> MTTLRAFTCDDLFRFNNINLDPLTETYGIPFYLQYLAHWPEYFIVAEAPGGELMGYIMGKAEGSVAREEWHGHVTALSVAPEFRRLGLAAKLMELLEEISERKGGFFVDLFVRVSNQVAVNMYKQLGYSVYRTVIEYYSASNGEPDEDAYDMRKALSRDTEKKSIIPLPHPVRPEDIE;> MATRGHVQDPNDRRLRPIYDYLDNGNNKMAIQQADKLLKKHKDLHCAKVLKAIGLQRTGKQEEAFTLAQEVAALEPTDDNSLQALTILYREMHRPELVTKLYEAAVKKVPNSEEYHSHLFMAYARVGEYKKMQQAGMALYKIVPKNPYYFWSVMSLIMQSISAQDENLSKTMFLPLAERMVEKMVKEDKIEAEAEVELYYMILERLGKYQEALDVIRGKLGEKLTSEIQSRENKCMAMYKKLSRWPECNALSRRLLLKNSDDWQFYLTYFDSVFRLIEEAWSPPAEGEHSLEGEVHYSAEKAVKFIEDRITEESKSSRHLRGPHLAKLELIRRLRSQGCNDEYKLGDPEELMFQYFKKFG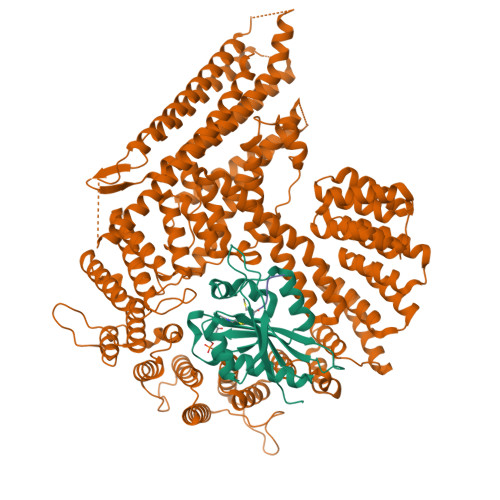DKPCCFTDLKVFVDLLPATQCTKFINQLLGVVPLSTPTEDKLALPADIRALQQHLCVVQLTRLLGLYHTMDKNQKLSVVRELMLRYQHGLEFGKTCLKTELQFSDYYCLLAVHALIDVWRETGDETTVWQALTLLEEGLTHSPSNAQFKLLLVRIYCMLGAFEPVVDLYSSLDAKHIQHDTIGYLLTRYAESLGQYAAASQSCNFALRFFHSNQKDTSEYIIQAYKYGAFEKIPEFIAFRNRLNNSLHFAQVRTERMLLDLLLEANISTSLAESIKSMNLRPEEDDIPWEDLRDNRDLNVFFSWDPKDRDVSEEHKKLSLEEETLWLRIRSLTLRLISGLPSLNHPVEPKNSEKTAENGVSSRIDILRLLLQQLEATLETGKRFIEKDIQYPFLGPVPTRMGGFFNSGCSQCQISSFYLVNDIYELDTSGLEDTMEIQERIENSFKSLLDQLKDVFSKCKGDLLEVKDGNLKTHPTLLENLVFFVETISVILWVSSYCESVLRPYKLNLQKKKKKKKETSIIMPPVFTSFQDYVTGLQTLISNVVDHIKGLETHLIALKLEELILEDTSLSPEERKFSKTVQGKVQSSYLHSLLEMGELLKKRLETTKKLKI;> MDVFM> MSALRVTSPSVEYVQRPLGLDAAHPRLSWPMASAAPGRRQSAYQVRVASSAAGLSHPDVWDSGKVVSDDSVLVPYAGPPLKPRTRYFWSVRVWDADGGASEWSAPSWWETGLMGASQWSAKWISAPAPLTEAPSLEGSSWIWFPEGEPANSAPAATRWFRRTVDLPDDITGATLAISADNVYAVSVDGAEVARTDLEADNEGWRRPAVIDVLDHVHSGNNTLAVSASNASVGPAGWICVLVLTTASGEKKIFSDASWKSTDHEPADGWREPDFDDSGWPAAKVAAAWGAGPWGRVAPVASAANQLRHEFRLPHKKVSRARLYATALGLYEAHLNGRRVGRDQLAPGWTDYRKRVQYQTYDVTSSVRPGANALAAYVAPGWYAGNVGMFGPHQYGERPALLAQLEVEYADGTSERITSGPDWRAASGPIVSADLLSGETYDARKETAGWTSPGFDDRAWLAVRGADNDVPEQIVAQVDGPVRIAKELPARKVTEPKPGVFVLDLGQNMVGSVRLRVSGDAGTTVRLRHAEVLNPDGTIYTANLRSAAATDTYTLKGQGEETYEPRFTFHGFRYVEVTGFPGKPSTTSVTGRVMHTSAPFTFEFETNVPMLNKLHSNITWGQRGNFLSVPTDTPARDERLGWTGDINVFAPTAAYTMESARFLTKWLVDLRDAQTSDGAFTDVAPAVGNLGNGVAGWGDAGVTVPWALYQAYGDRQVLADALPSVHAWLRYLEKHSDGLLRPADGYGDWLNVSDETPKDVIATAYFAHSADLAARMATELGKDAAPYTDLFTRIRKAFQTAYVASDGKVKGDTQSAYVLTLSMNLVPDALRKAAADRLVALIEAKDWHLSTGFLGTPRLLPVLTDTGHTDVAYRLLHQRTFPSWGYPIDKGSTTMWERWDSIQPDGGFQTPEMNSFNHYAYGSVGEWMYANIAGIAPGRAGYRQVVIRPRPGGE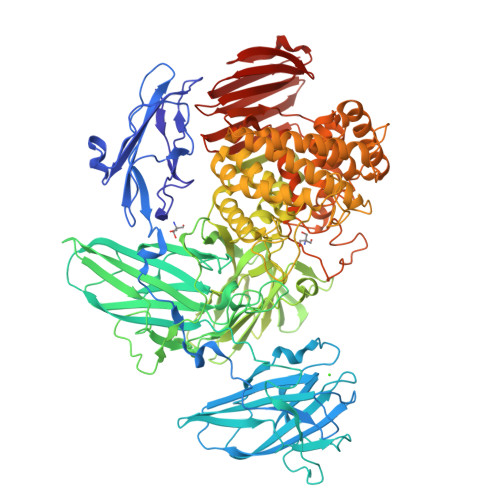VTSARATFASLHGPVSTRWQQRSGGFVLTCSVPPNTTAEVWIPADHPDRVQHTHGTFVRAEDGCAVFEVGSGSHRFTVKLAAALEHHHHHH>[2x]MALEEIRPKEVYLDRKLL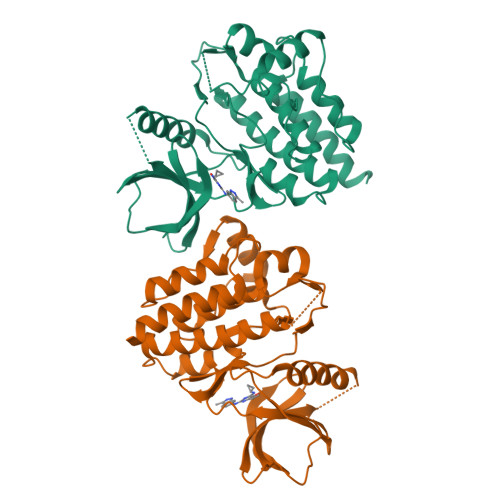TLEDKELGSGNFGTVKKGYYQMKKVVKTVAVKILKNEANDPALKDELLAEANVMQQLDNPYIVRMIGICEAESWMLVMEMAELGPLNKYLQQNRHVKDKNIIELVHQVSMGMKYLEESNFVHRDLAARNVLLVTQHYAKISDFGLSKALRADENYYKAQTHGKWPVKWYAPECINYYKFSSKSDVWSFGVLMWEAFSYGQKPYRGMKGSEVTAMLEKGERMGCPAGCPREMYDLMNLCWTYDVENRPGFAAVELRLRNYYYDVVNEGHHHHHH>[6x]MSSAVDNINKTIRDFET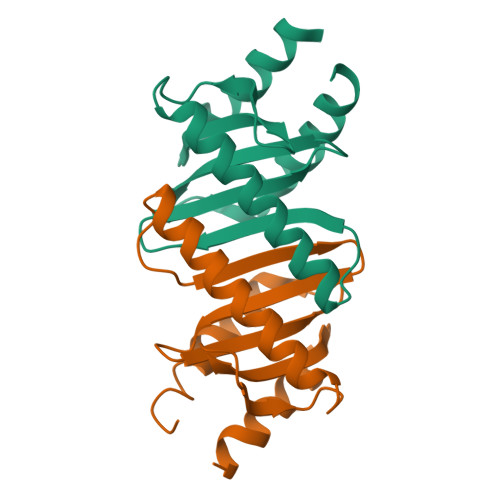VPGVEGAALVSADGLMISSALPETEQERVAAISAGLLSLGEKATTELDRGNFKEVYVKGEKGYTLLTSVGENALLLVLAKADAQIGLIFVDMRRIADSLLEIL> MSLQENISVTDSYSTGNAAQAMLEKLLQIYDVKMLVAQLNGVGENHWSAAILKRALANDSAWHRLSEKEFAHLQTLLPKPPEHHPHYAFRFIDLFAGIGGIRRGFESIGGQCVFTSEWNKHAVRTYKANHYCDPATHHFNEDIRDITLSHQEGVSDEAAAEHIRQHIPEHDVLLAGFPCQPFSLAGVSKKNSLGRAHGFACDTQGTLFFDVVRIIDARRPAMFVLENVKNLKSHDKGKTFRIIMQTLDELGYDVADAEDNGPDDPKIIDGKHFLPQHRERIVLVGFRRDLNLKADFTLRDISECFPAQRVTLAQLLDPMVEAKYILTPVLWKYLYRYAKKHQARGNGFGYGMVYPNNPQSVTRTLSARYYKDGAEILIDRGWD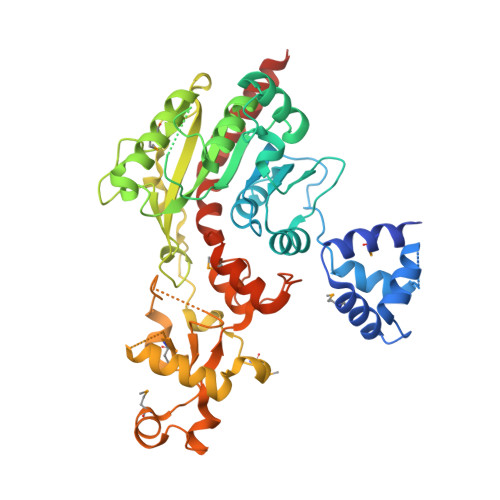MATGEKDFDDPLNQQHRPRRLTPRECARLMGFEAPGEAKFRIPVSDTQAYRQFGNSVVVPVFAAVAKLLEPKIKQAVALRQQEAQHGRRSREGHHHHHH>[2x]MAKHPTPMLDELEKGPWPSFVSDIKQECDNRAKNPKGLDYQIPAECPDDLLGILELSFHEGETHWKHGGIVGVFGYGGGVIGRYCDQPEMFPGVAHFHTVRLAQPAAKYYTAEYLEAICDVWDLRGSGLTNMHGSTGDIVLLGTQTPQLEEIFFEMTHNLNTDLGGSGSNLRTPESCLGISRCEFACYDTQLMCYQLTQDYQDELHRPAFPYKFKFKFDGCPNGCVASMARSDFAVIGTWKDDIKIDQEAVKAYVGGEFKPNAGAHAGRDWGKFDIEAEVVGLCPTGCMTYESGTLSIDNKNCTRCMHCINTMPRALKIGDERGASILVGAKAPVLDGAQMGSLLIPFIAAEEPFDEVKEVIENIWEWWMEEGKNRERLGETMKRVGFQKLLEVTGTKAVPQHVSEPRHNPYIFFKEEEVPGGWSRDISDYR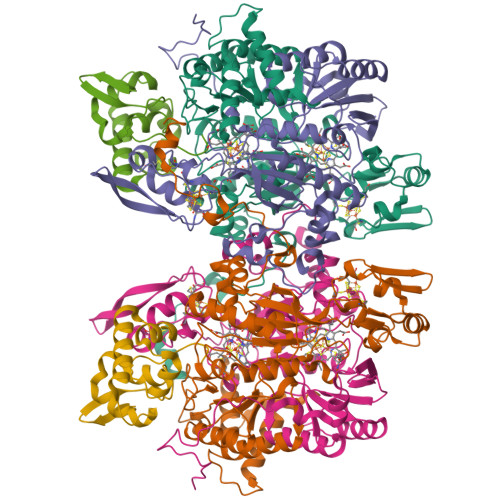KRHMR;>[2x]MAFISSGYNPAKPMENRITDIGPRKFTEFFPPVIAKNAGNWDYHEILEPGILVHVAKNGDKVFTVRCGAARLMSTSHIREACEIAKKFCNGHLRFTTRNNIEFMVDNEETLKALVADLKTRKFAAGSFKFPIGGTGASISNIVHTQGWVYCHTPATDASGPVKAVMDELFEEFTSMRLPAIVRVSLACCINMCGAVHCSDIGLVGIHRKPPMIDHENLAELCEIPLAVAACPTAAVKPITAEVNGQKVKSVAINNDRCMYCGNCYTMCPALPLSDGTGDGIAIMVGGKISNRIKVPSFSKVVVAFVPNEPPRWPTMAKIVKKIVEVYAEDARKYERIGDWIHRIGWETFYEKTGLEFSHHCIDDFRDPAYYTWRQSTQFKFVSFDS;>MAVVEFAGSAFEVDEDGFLNAFDDWCPEWVKYAKGSEGIGAGSADHQKIIDFLQDYYKANGIAPMVRILSKNTGFALKEIYELFPSGPGKGACKMAGLPKPTGCV[2x]>GSHMVKLSSKNLDARLDTVYDAIVLGGGMGGLSAAIYLARYGLKCLVVEKGRGRSFWMQDLRNYVGLDPDTPGRDIITHSTQQALHWGADLLRGYVEDVTDEGDTLAVKVKVGKKDSLYPIFRTKYVIAATGIIDNLPQLEDMQNVYDYAGYTLHVCMICDGFDMWDQKAVLIAGTEGQINAAFVLNWFTPYITVLTHGLCTVGDEMKAKLADHGYPLHEAAITKFLGEDHKMSGVELVDGTVMEATTGLINMGSVYHNHYLKG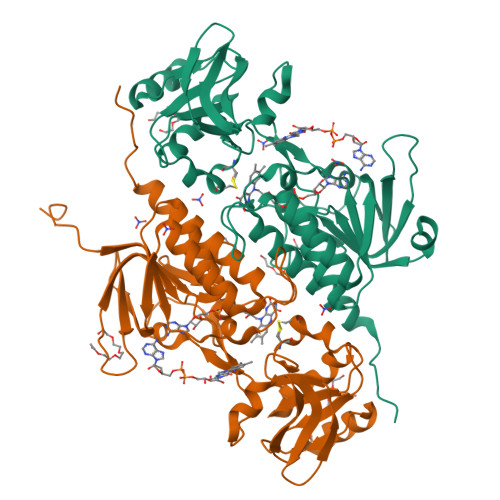IEGLEWDGENLVTNDMAQTSHPRIFALGDLKKGLNQVSVAVADGTLAATQIWRNIRRASEPRKWIH[4x]>YLEAFPKELREYYKNLFGKEEANKIMKKLREPVEHYYIRVNTLKISREKLIGELKKEGLKPLRSPYLPEGLYFVREGPNFSDDFEPKLPVVVANKYAAESVYQGAMLYAPGVLKADKNIKEGDEVQIRDPKGLLVGIGIARMDYKEMTEATRGLAVEVTLPKFKLPSLSELKAFEKGYFYPQGLPSMVTARVLEPKEDDVIIDMAAAPGGKTTHIAQLLENKGEIIAIDKSKNRLRKMEENIKRLGVKNVKLVQMDARKLPDLGIKADKILLDAPCTALGVRPKLWEERTLKHIEATARYQRAFIWAAIKSLRRGGVLVYSTCTLSYEENEGNVKFMIRKGMKLEEQSIFIGSPGIGMNKVQR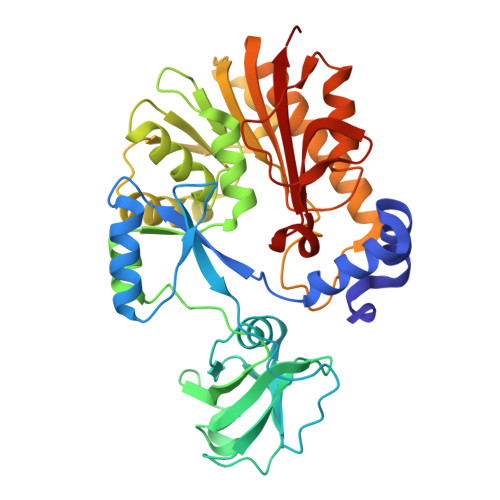FYPHKHLTQGFFIAKLRKVKD[2x]~{N}-[5-[2-azanyl-5-(4-piperazin-1-ylphenyl)pyridin-3-yl]-2-methoxy-phenyl]propane-1-sulfonamide | C25 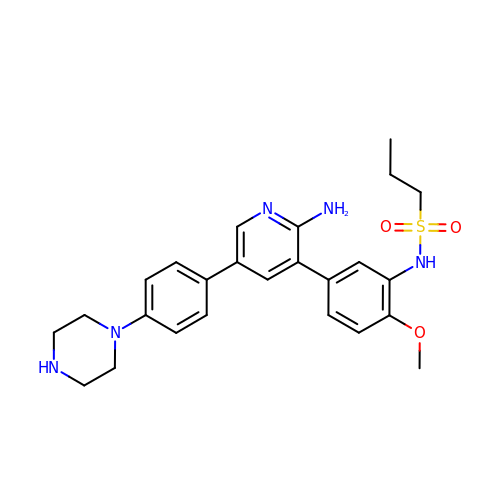H31 N5 O3 S | JMJHOMFUECZGAD-UHFFFAOYSA-N> MGSMELLEYIKREQERWDSETKSVSDSSRDTGRGVKYWFCYGTKCYYFIMNKTTWSGCKANCQHYSVPIVKIEDEDELKFLQRHVILESYWIGLSYDKKKKEWAWIHNGQSKLDMKIKKMNFTSRGCVFLSKARIEDTDCNT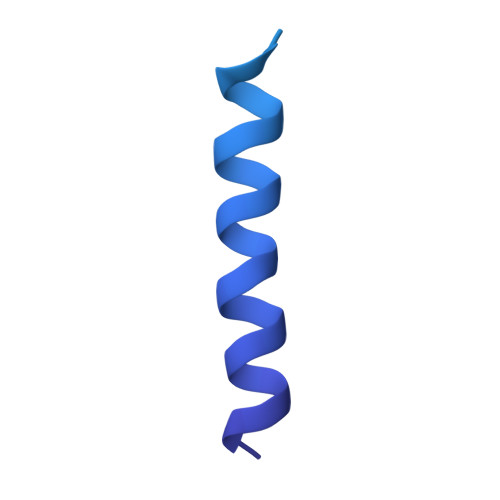PYYCICGKKLDKFPD> MDDLVFAGNKALYLVLILSGWPTIVATIIGLLVGLFQTVTQLQEQTLPFGIKLLGVCLCLFLLSGWYGEVLLSYGRQVIFLA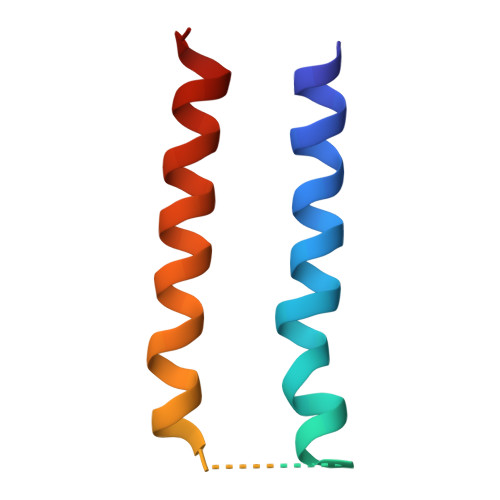LAKG Myo7 is a crucial component of the tripartite complex that maintains the necessary mechanical tension across the cadherin links. The Myo7 tail domain consists of two MyTH4-FERM (MF; myosin tail homology 4; band 4.1, ezrin, radixin, moesin) domains separated by an SH3 domain. Harmonin plays a pivotal role due to its ability to interact with cadherin as well as all other components of the complex. The results presented here reveal nearly identical interactions between members of the Myo7/harmonin-a/SANS:ANKS4B tripartite complexes that link cadherins to the actin-rich core in stereocilia and microvilli. Both Myo7a and Myo7b MF2 domains bind to harmonin-a PDZ3c with similar affinities via a novel mode.

The basis of the harmonin-a PDZ3c/Myo7b MF2 interaction was determined by solving the crystal structures of Myo7b MF2 and of PDZ3c/Myo7b MF2 complex at 2.44 and 1.88 Å resolution, respectively. The MF2 domain adopts a canonical MyTH4-FERM supramodule, with limited flexibility between the MyTH4 and FERM domains; while the FERM domain consists of three globular subdomains or ‘lobes’, similar to previously described MF structures. Limited structural changes are found in the Myo7b MF2 supramodule upon PDZ3c binding, with an overall r.m.s.d. of 0.63 Å for 414 Cα atoms between the bound and free structures. This limited conformational pliability upon cargo binding indicates that the groove of a particular FERM domain defines its cargo recognition. The five linkers in the FERM lobes dictate the orientation of each lobe and thus define the shape and, as a result, the specificity of the central groove. The distinct orientation of the FERM lobes in Myo7b MF1 and MF2 domains readily explains their specific recognition of different targets within their FERM core elements (reviewed in27).

> HHHHHHSSGHKEKLHTLEEFSYEFFRAPEKDAVSMAVLPLARARGHLWAYSCEPLRQPLLKRVHANVDLWDIACQIFVAILRYMGDYPSRQAWPTLELTDQIFTLALQHPALQDEVYCQILKQLTHNSNRHSEERGWQLLWLCTGLFPPSKGLLPHAQKFIDTRRGKLLAPDCSRRIQKVLRTGPRKQPPHQVEVEAAEQNVSRICHKIYFPNDTSEMLEVVANTRVRDVCDSIATRLQLASWEGCSLFIKISDKVISQKEGDFFFDSLREVSDWVKKNKPQKEGAPVTLPYQVYFMRKLWLNISPGKDVNADTILHYHQELPKYLRGFHKCSREDAIHLAGLIYKAQFNNDRSQLASVPKILRELVPENLTRLMSSEEWKKSILLAYDKHKDKTVEEAKVAFLKWICRWPTFGSAFFEVKQTSEPSYPDVILIAINRHGVLLIHPKTKDLLTTYPFTKISSWSSGSTYFHMALGSLGRGSRLLCETSLGYKMDDLLTSYVQQLLSAMNKQRGSKAPALAST>ENLMQVYQQARLSNPELRKSAADRDAAFEKINEARSPLLPQLGLGADYTYSNGYRDANGINSNETSASLQLTQTLFDMSKWRGLTLQEKAAGIQDVTYQTDQQTLILNTANAYFKVLNAIDVLSYTQAQKEAIYRQLDQTTQRFNVGLVAITDVQNARAQYDTVLANEVTARNNLDNAVEELRQVTGNYYPELASLNVEHFKTDKPKAVNALLKEAENRNLSLLQARLSQDLAREQIRQAQDGHLPTLNLTASTGISDTSYSGSKTNSTQYDDSNMGQNKIGLNFSLPLYQGGMVNSQVKQAQYNFVGASEQLESAHRSVVQTVRSSFNNINASISSINAYKQAVVSAQSSLDAMEAGYSVGTRTIVDVLDATTTLYDAKQQLANARYTYLINQLNIKYALGTLNEQDLLALNSTLGKPIPTSPESVAPETPDQDAAADGYNAHSAAPAVQPTAARANSNNGNPFRH[3x]

ST50, an outer-membrane protein with the molecular mass of approximately 50 kDa, is expected to be a tripartite member of the resistance-nodulation-cell division (RND) efflux system because of its high sequence identity with TolC (89%), one component of the drug efflux system AcrA-AcrB-TolC in E. coli. ST50, similar to other outer-membrane proteins involved in resistance-nodulation-cell division (RND) efflux systems, possesses an α-helical barrel domain, a membrane-embedded β-barrel domain and an equatorial domain of mixed α/β-structures. One outer-membrane component of the heavy metal efflux pump, CusC, also possesses an architecture similar to those of the outer-membrane multidrug efflux pumps. These tripartite efflux pumps are able to transport diverse substrates, including metal ions, dyes, detergents, antibiotics and protein toxins, from the cytoplasm to the external medium of the microorganism. Currently, the principal method to diagnose typhoid fever is TYPHIDOT, a rapid immunoassay test to detect IgM and IgG antibodies against the outer-membrane protein ST50 of S. Typhi.

To identify the immunogenic site of ST50 and investigate the structural features of this antigenic outer-membrane protein, we overexpressed ST50 from Salmonella enterica serovar Typhi in E. coli and determined its structure at a resolution of 2.98 Å. In one asymmetric unit, three protomers of ST50 form a functional trimer through interactions of the interprotomer H7/(adjacent H2, H4) coiled-coil and the antiparallel β-sheet S5/(adjacent S1). The long extracellular loops L2 between β-strands S4 and S5 exhibit varied conformations among the three protomers, and the B-chain possesses the largest conformational deviation. The distinct conformation and the large temperature factor of the L2 loop in the B protomer result from compression on the L2 loop by helix 1 of another adjacent ST50 molecule that is related to crystal packing (θ/A-protomer = 103.1°, θ/C-protomer = 100.2°, θ/B-protomer = 71.8°). The periplasmic entrance of ST50 adopts the resting closed state through close interactions between the α-helical inner coiled-coil (H7/H8) and the outer coiled-coil (H3/H4) through hydrogen bond networks, similar to those of TolC, Oprm and VceC8910. The hydrogen bond network comprises four key residues: Thr152, Asp153, Tyr359 and Arg364 in ST50, corresponding to Thr152, Asp153, Tyr362 and Arg367 in TolC. Four bound detergent molecules of n-octyl-β-D-glucoside (β-OG) are found in the structure of ST50. His244 of all three ST50 protomers interact with the β-OG molecules through hydrogen bonding between the imidazole ring of His244 and the polar group of β-OG. Our structure reveals that one β-OG molecule is bound at the D-cage, which comprises three sets of Asp368 and Asp371 residues, at the entrance of the periplasmic tunnel.>SADVAGAVIDGAGLGFDVLKTVLEALGNVKRKIAVGIDNESGKTWTAMNTYFRSGTSDIVLPHKVAHGKALLYNGQKNRGPVATGVVGVIAYSMSDGNTLAVLFSVPYDYNWYSNWWNVRVYKGQKRADQRMYEELYYHRSPFRGDNGWHSRGLGYGLKSRGFMNSSGHAILEIHVTK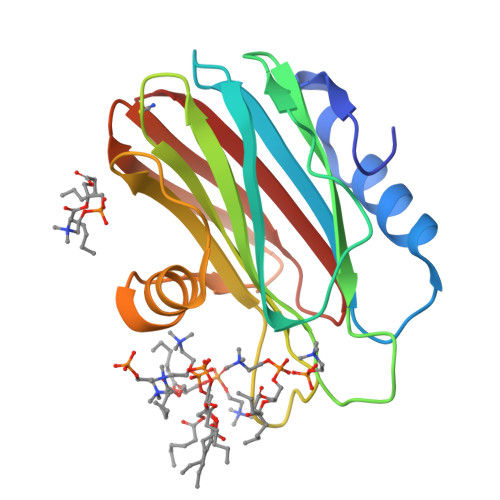A[6x]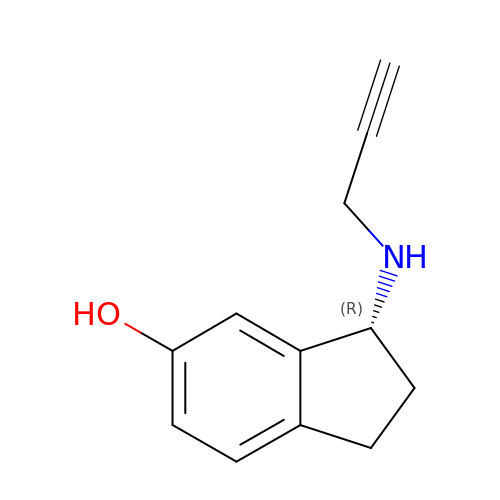(3R)-3-(PROP-2-YNYLAMINO)INDAN-5-OL | C12 H13 N O | NRSDGDXUWMMUEV-GFCCVEGCSA-N> APITAYAQQTRGLLGCIITSLTGRDKNQVEGEVQIMSTATQTFLATCINGVCWTVY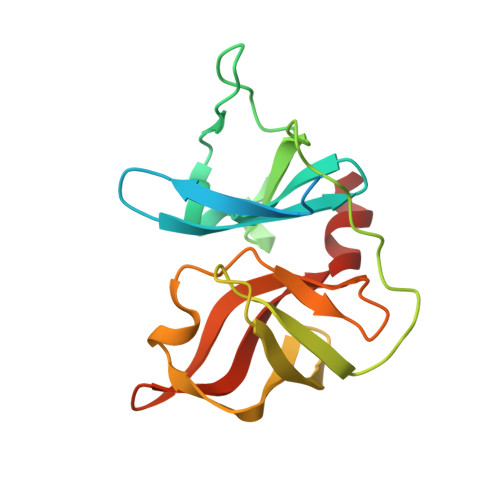HGAGTRTIASPKGPVIQMYTNVDQDLVGWPAPQGSRSLTPCTCGSSDLYLVTRHADVIPVRRRGDSRGSLLSPRPISYLKGSSGGPLLCPAGHAVGLFRAAVCTRGVAKAVDFIPVENLETTMRS>MGSSHHHHHHSSGLVPRGSHMASATASRGASQAGAPQGRVPEARPNSMVVEHPEFLKAGKEPGLQIWRVEKFDLVPVPTNLYGDFFTGDAYVILKTVQLRNGNLQYDLHYWLGNECSQDESGAAAIFTVQLDDYLNGRAVQHREVQGFESATFLGYFKSGLKYKKGGVASGFKHVVPNEVVVQRLFQVKGRRVVRATEVPVSWESFNNGDCFILDLGNNIHQWCGSNSNRYERLKATQVSKGIRDNERSGRARVHVSEEGTEPEAMLQVLGPKPALPAGTEDTAKEDAANRKLAKLYKVSNGAGTMSVSLVADENPFAQGALKSEDCFILDHGKDGKIFVWKGKQANTEERKAALKTASDFITKMDYPKQTQVSVLPEGGETPLFKQFFKNWRDPDQTDGLGLSYLSSHIANVERVPFDAATLHTSTAMAAQHGMDDDGTGQKQIWRIEGSNKVPVDPATYGQFYGGDSYIILYNYRHGGRQGQIIYNWQGAQSTQDEVAASAILTAQLDEELGGTPVQSRVVQGKEPAHLMSLFGGKPMIIYKGGTSREGGQTAPASTRLFQVRANSAGATRPVEVLPKAGALNSNDAFVLKTPSAAYLWVGTGASEAEKTGAQELLRVLRAQPVQVAEGSEPDGFWEALGGKAAYRTSPRLKD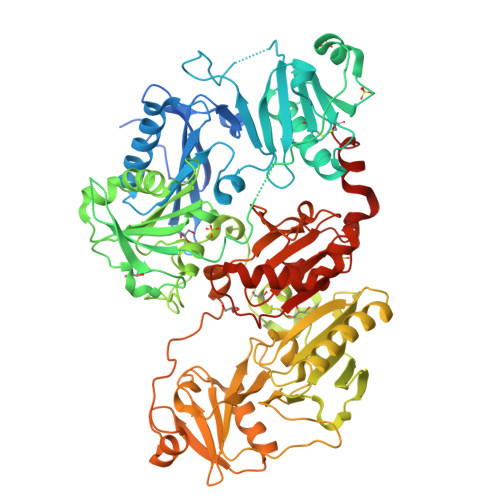KKMDAHPPRLFACSNKIGRFVIEEVPGELMQEDLATDDVMLLDTWDQVFVWVGKDSQEEEKTEALTSAKRYIETDPANRDRRTPITVVKQGFEPPSFVGWFLGWDDDYWSVDPLDRAMAELAA[2x]>[4x]MHHHHHHSIEGRPHMDFKNINLGIFGHIDHGKTTLSKVLTEIASTSAHDKLPESQKRGITIDIGFSAFKLENYRITLVDAPGHADLIR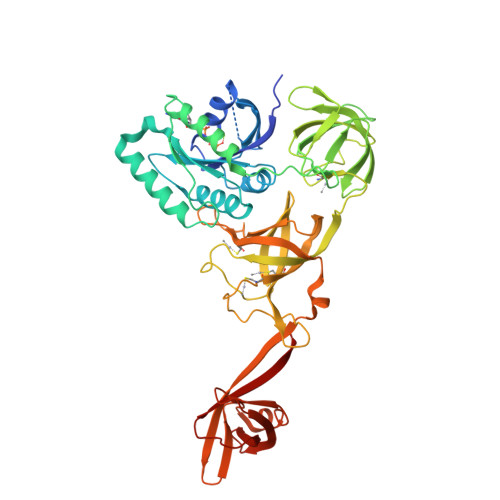AVVSAADIIDLALIVVDAKEGPKTQTGEHMLILDHFNIPIIVVITKSDNAGTEEIKRTEMIMKSILQSTHNLKNSSIIPISAKTGFGVDELKNLIITTLNNAEIIRNTESYFKMPLDHAFPIKGAGTVVTGTINKGIVKVGDELKVLPINMSTKVRSIQYFKESVMEAKAGDRVGMAIQGVDAKQIYRGCILTSKDTKLQTVDKIVAKIKISDIFKYNLTPKMKVHLNVGMLIVPAVAVPFKKVTFGKTEENIILNEVISGNECYCAFELEEKVLAEVGDRVLITRLDLPPTTLRICGHGLIEEFKPIKDLNIKKEVLREGKVKIDKGRTVIDGLAQSKVAAEKLIGEEISIEGKDIVGKIKGTFGTKGLLTAEFSGNVENRDKVILNRLRRWG> MAIAFEHVTYTYQAGTPMAHTALTDVSLTVPDRGYLAIIGHTGSGKSTLIQQLNALLKPTSGTIKIDEFTITPETTNAALKPLRQHVGMVFQFPENQLFEETVRQDIAFGPKNFGMADADALALADEMLTTVGLDQSYAERSPFELSGGQMRRVAIAGVLAMQPKVLVLDEPTAGLDPQGRQEMMRLFARLHQEQGLTIVLVTHQMEDVAQYAEQVAVMHEGRLMKFGTPADVFSNREWLQDHQLDVPQAAQFARRLRDRGLTFPKQPLTADQLADYLAQQWAQRGADHV;> MTENIISVDHLTYQYDENQAPALTDVSFTVHAGEWLAIVGHNGSGKSTLAKSLDGLLPFTQGSVTVGGITLTPETVWQVREQIGMIFQNPDNQFVGATVEDDVAFGLENRQISRDEMVPRVQAALAQVGMTSFAQREPSSLSGGQKQRVALAGIVA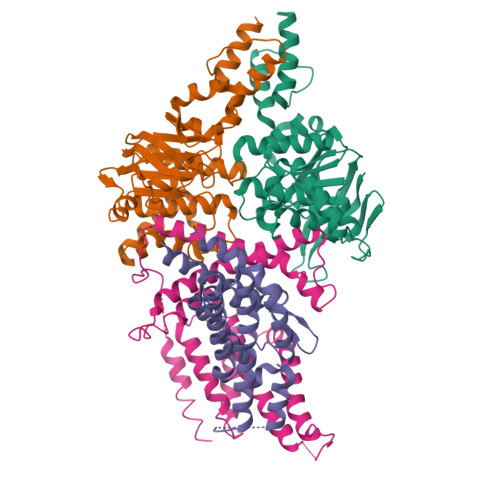IAPKILILDEATSMLDPQGRIEMLAIVRQLRQQQNLTVISITHDIDEAASADRVLVIDDGRLVDEAVPSQIFERGTQLVEMGLDLPFTEKLKAALRQRGITPPTTYQTAAEMEEWLWQSLSNT;> MTRHKTFRLVVDALLMAIVLLQNLVPFLGYIPFGPFSMTLIGLTVIVAGSALGPRDGLLIGGFWGLITFVRAFTWPSSPVAPLIFTNPLISILPRLLMGLVAGSLYLWGRHRQWSMRQAMQVAAGCAALTNTVLVLGLVFLFYQTPAVATAFGATGNQTLGYVLMISLFTNGIPELILDVLVAPLIAMPLRRQWERLKPQTTK;> MGSSHHHHHHSQDPMSNFIFGRYLPLDSVVHRLDPRAKLMLSFCYIIVVFLANNIWSYAILIAFTVGAILSSKISLGFFLKGIRPLLWLIVFTVVLQLLFSPAGGHTYFHWAFINVTQDGLINAGYIFVRFLLIIMMSTLLTLSTQPLDIATGLASLMKPLRWVKVPVDTLAMMLSIALRFVPTLMDEATKIMNAQRARGVDFGEGGLFKQAKSLIPLMVPLFMSAFNRAEDLSTAMEARGYQDSEHRSQYRILTWQRRDTVTWLLFLLGFVAILIFRHW2-(4,6-dimethylpyrimidin-2-yl)sulfanyl-N-[3-(phenoxymethyl)phenyl]ethanamide | C21 H21 N3 O2 S | 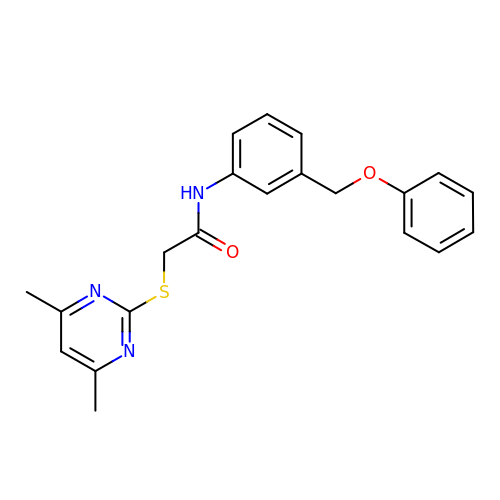UTHZHWWWTOWRMG-UHFFFAOYSA-N> MASPAVRKAISDAALQYAKPEGKIFQYGTAGFRMKADLLNTVVYAVGLLATLRSKKLSGQWIGVMVTAAHNPAEDNGVKLVDPMGEMLEAEWEAYATKLANAPLENIGDVYDELVKEIDVSMENPARVVFARDTRASGSRLIGVLSAALTATEAEFIDMKFMTTPQLHYVVRCKNTLGTQYEYGEPTEQGYYEKLAAAFKRVMRGVKVKGSLTVDCANGVGGPKLRELIKYLPEDTGLDIKIVNDDVINPDSLNFECGADYVKTKQRAPPSSKASILDRCASLDGDADRILYYFLDEGNVFRLLDGDRIATLAASFIGDLARSAGIAQKLKIGVVQTAYANGSSTEYIEKVLKLPSVCTNTGVKHLHHAA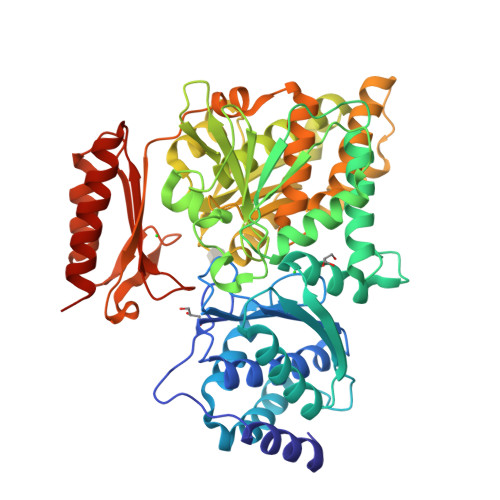MRFDVGVYFEANGHGTITFSENALKTIKNTEPQSPAQQRSLECLQALTDLINQAVGDAISDMLLVEAILAHKGWTPKEWLATYTDLPSRLVRVEVAERSIFKAYDAERKLESPPGLQAKIDSLQSRYNKGRSFARASGTEDAVRVYAEAASRSEADDLATRVANAVRDAGTVKEILQAS>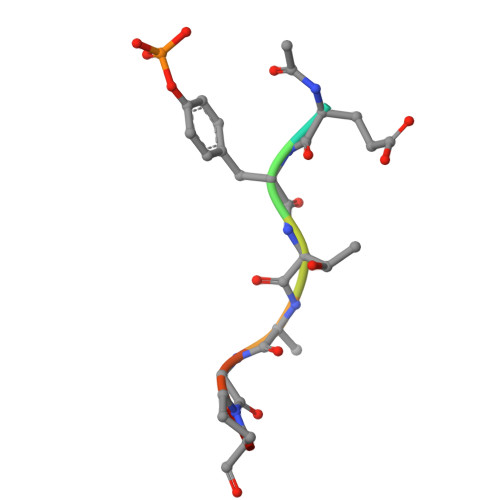 XEYTEGPT(3~{S},4~{S})-4,5,5-tris(oxidanyl)piperidine-3-carboxylic 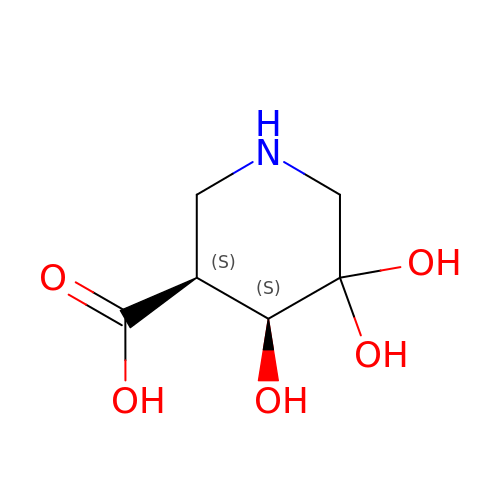acid | C6 H11 N O5 | VJJFPBNJYGLWRR-IMJSIDKUSA-N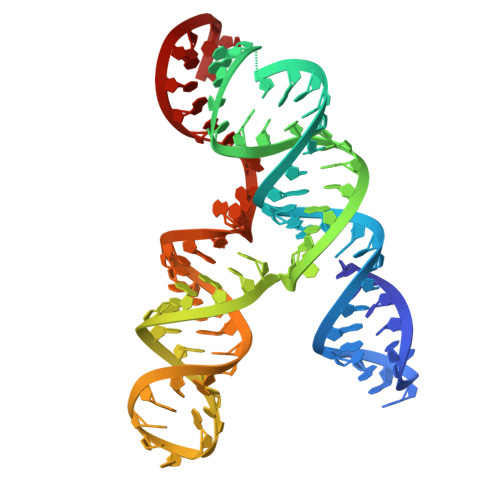> GUUUUUAAACGGGUUUGCGGUGUAAGUGCAGCCCGUCUUACACCGUGCGGCACAGGCACUAGUACUGAUGUCGUAUACAGGGCUUUUG> AALAEIVAQLNIYQSQVELIQQQMEAVRATISELEILEKTLSDIQGKDGSETLVPVGAGSFIKAELKDTSEVIMSVGAGVAIKKNFEDAMESIKSQKNELESTLQK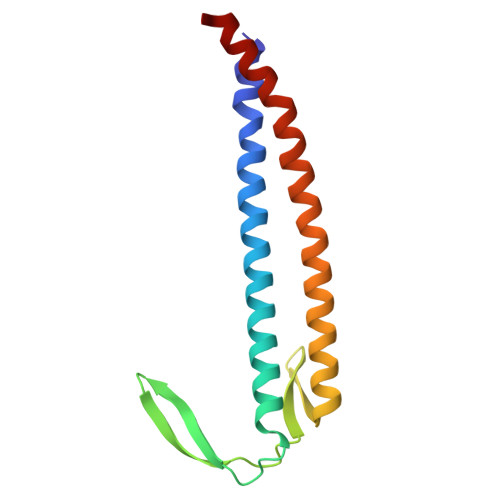MGENLRAITDIMMKLSPQAEELLAAVA> SAEACGYSDRVAQLTLGNSTITTQEAANIVVGYGRWPTSLRDTDATAVDKPTQPGVSAERFYTLPS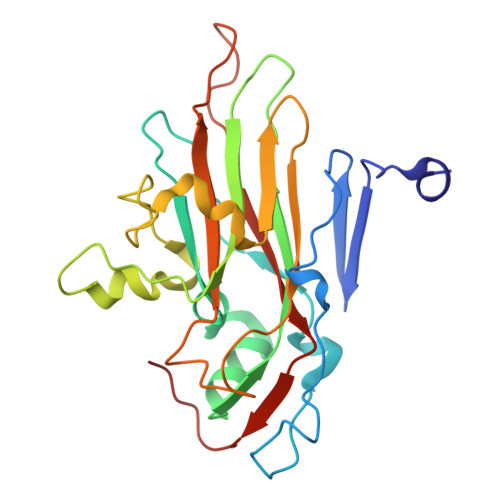VQWTNSFKGHYWKLPDALSELGLFGQNLQFHYLYRGGWVIHVQCNATKFHQGTLLVVATPEHKIQSAESPAFARTNPGEQGAAYQFPFTFEDGTALGNALIYPHQWVNLRTNNSATLVLPYVNALPMDSGIRHNNWTLSVIPIVPLEYAAGATTYVPITVTIAPMCTEYNGLRAAVTQ>[3x]MDFSKLPKIRDEDKESTFGYVHGVSGPVVTACDMAGAAMYELVRVGHSELVGEIIRLEGDMATIQVYEETSGVSVGDPVLRTGKPLSVELGPGIMGAIFDGIQRPLSDISSQTQSIYIPRGVNVSALSRDIKWEFIPSKNLRVGSHITGGDIYGIVNENSLIKHKIMLPPRSRGSVTYIAPPGNYDASDVVLELEFEGVKEKLSMVQVWPVRQVRPVTEKLPANHPLLTGQRVLDALFPCVQGGTTAIPGAFGCGKTVISQSLSKYSNSDVIIYVGCGERGNEMSEVLRDFPELTMEVDGKVESIMKRTALVANTSNMPVAAREASIYTGITLSEYFRDMGYHVSMMADSTSRWAEALREISGRLAEMPADSGYPAYLGARLASFYERAGRVKCLGNPEREGSVSIVGAVSPPGGDFSDPVTSATLGIVQVFWGLDKKLAQRKHFPSVNWLISYSKYMRALDEYYDKHFTEFVPLRTKAKEILQEEEDLAEIVQLVGKASLAETDKITLEVAKLIKDDFLQQNGYTPYDRFCPFYKTVGMLSNMISFYDMARRAVETTAQSDNKITWSIIREHMGEILYKLSSMKFKDPVKDGEAKIKADYAQLLEDMQNAFRSLED;>[3x]MALRAMRGIVNGAAPELPVPTGGPMAGAREQALAVSRNYLSQPRLTYKTVSGVNGPLVILDHVKFPRYAEIVHLTLPDGTKRSGQVLEVSGSKAVVQVFEGTSGIDAKKTSCEFTGDILRTPVSEDMLGRVFNGSGKPIDRGPVVLAEDFLDIMGQPINPQCRIYPEEMIQTGISAIDGMNSIARGQKIPIFSAAGLPHNEIAAQICRQAGLVKKSKDVVDYSEENFAIVFAAMGVNMETARFFKSDFEENGSMDNVCLFLNLANDPTIERIITPRLALTTAEFLAYQCEKHVLVILTDMSSYAEALREVSAAREEVPGRRGFPGYMYTDLATIYERAGRVEGRNGSITQIPILTMPNDDITHPIPDLTGYITEGQIYVDRQLHNRQIYPPINVLPSLSRLMKSAIGEGMTRKDHADVSNQLYACYAIGKDVQAMKAVVGEEALTSDDLLYLEFLQKFEKNFITQGPYENRTVYETLDIGWQLLRIFPKEMLKRIPQSTLSEFYPRDSAKH;> MSGKDRIEIFPSRMAQTIMKARLKGAQTGRNLLKKKSDALTLRFRQILKKIIETKMLMGEVMREAAFSLAEAKFTAGDFSTTVIQNVNKAQVKIRAKKDNVAGVTLPVFEHYHEGTDSYELTGLARGGEQLAKLKRNYAKAVELLVELASLQTSFVTLDEAIKITNRRVNAIEHVIIPRIERTLAYIITELDEREREEFYRLKKIQEKKKIIKEKSEKDLERRRAAGEVMEPANLLAEEKDEDLLFE;>[3x]MALSDADVQKQIKHMMAFIEQEANEKAEEIDAKAEEEFNIEKGRLVQTQRLKIMEYYEKKEKQIEQQKKIQMSNLMNQARLKVLRARDDLITDLLNEAKQRLSKVVKDTTRYQVLLDGLVLQGLYQLLEPRMIVRCRKQDFP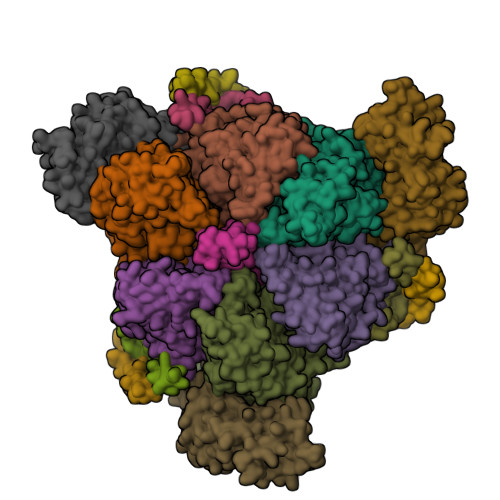LVKAAVQKAIPMYKIATKKDVDVQIDLEAYLPEDIAGGVEIYNGDRKIKVSNTLESRLDLIAQQMMPEVRGALFGANANRKFLD;>MASQSQGIQQLLQAEKRAAEKVADARKRKARRLKQAKEEAQMEVEQYRREREQEFQSKQQAAMGSQGNLSAEVEQATRRQVQGMQSSQQRNRERVLTQLLGMVCDVRPQVHPNYRITV[3x];>[3x]GMSFIKVGIKMGGLTSEQYHSQVVGKIGYIARCMQTIDPENNLKKIREDYQDVLIWAEKNYRFEEILEASKSGKCPNDLDALSRRSLILQELLRLVSSISPFKMKLDLIESQYEKMKQHVNLWKSDYHVKLNQLNQLTDYLKNAAPTPKNNFLRAMTSVLQMQIAQYGITEDNEGINQLFKLGLHLLAMANEKIDEQYHLFKGYVKDQPEESPFEGILPAEDQKILVKTMIDYAMPKLSSKVLQDKLSALSSSDVLTKTLLDSIDRIVKENEKLNALSKDYKDHDGDYKDHDIDYKDDDDK>[2x]MSWSRPEPGDWSSPAELAELQRARLPQVIAQALRSPFYAARYEGRTPPRTA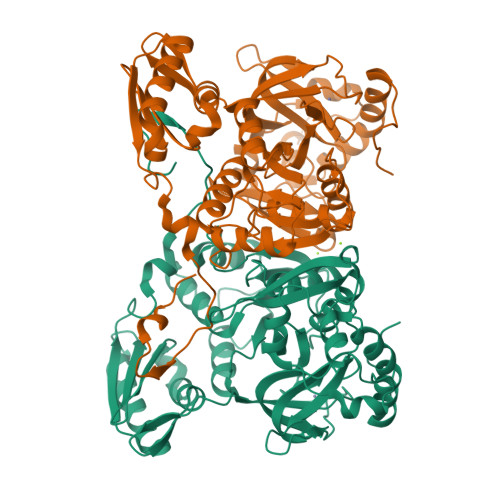DDFAGVELTTKQDLRDQYPFGMLAVERERLATYHESSGTAGDPTASYYTQEDWTDLAERFARKWTGIHPSDTFLVRTPYGLVITGHLAQAAGRLRGATVVPGDARSLATPLSRMVRVLKSLDVTLTWCNPTEITMLAAAAKAAGLRPDRDFPALRAMFTAAEPLTEVRRRRLSEIWGGVPVVEEYGSTETGTIAGQCPEGRMHLWADRAVFEVYDPATGELSEAGRGQMVVTPLYRDAMPLLRYNLADEVEVSTDPCPCGWLLPTVTVLGRAGTEHTVGSATVTQQRLEELVFSLPAAYEVMFWRAKAHPDVLHLQFEAPDATREQAAKELGAALDRELGVPHRIEGLPLGTLVPTEALTARRDILKARYLFAEGEDWDKAIMYF>MPVRRELADNATRGPTDGNYADELDVDVLIVGAGFGGIYSLYEMRKLGLKAVIYEAGNDIGGTWRWNCYPGAGVDSEVPEYQLSIPETWKDWTWSTNYPNYEDLRKYFDHVDKVLDIKKDCAFNSVVVGAHFHTVEGRWHIRTADGRTARAKYFIIAAGFAAKRYIPEWPGIEKFKGIVHHSSFWPDEKIDVRGKRCAIIGTGASGVQVTQAWGPEAGELKVFQRTPNLAVPMRKRSLTVEEQ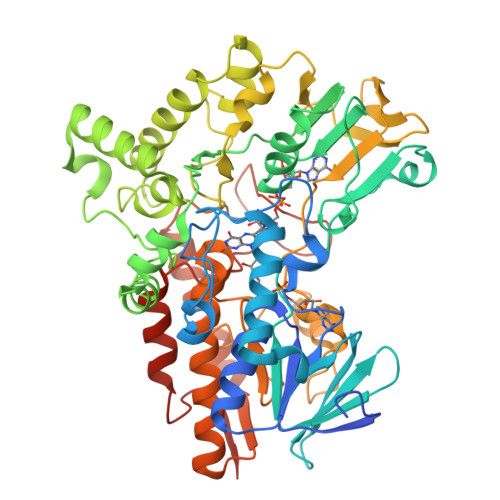EGAKAFYPELFRYREKCFAGFLYTWCERGVFEDSEEEREQFLEKLWSDGGFRYWVANYKDYLYDAKANRVVYDFWRKKVRERINDPKDQELLAPSEPPHPWGVKRPCLEYDYYEQFNRPNVDLVDIKDNSIVDFTEKGIKLQDGTEYEFDVVCIATGFDITTGGMTSMGLHSIHGDSLKEEWKSGAFTYLGMTVSGYPNMFHLYGPHGPTLLSNGPTTVEIQGRWIADAIKQMERQGIKYINPTAKAAKEWKAKINELSDKTLFPTTKSTYMGGSMPGKVFEQVNYAGGEYPYSKEIRAVLPNFNGFDIVKRHHHHHH[4x]> ALTQSVGGDSSADRLFPPQW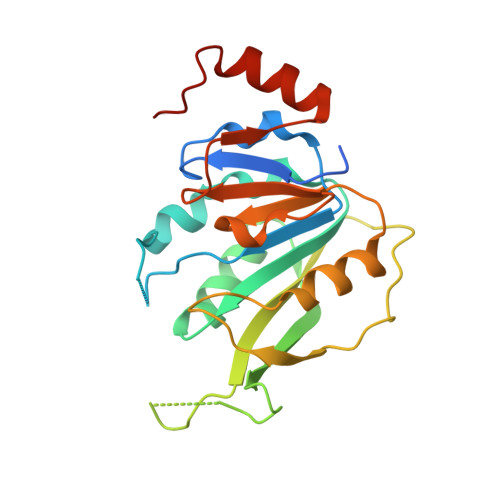ICCDIRYLDVSILGKFAVVMADPPWDIHMELPYGTLTDDEMRRLNIPVLQDDGFLFLWVTGRAMELGRECLNLWGYERVDEIIWVKTNQLQRIIRTGRTGHWLNHGKEHCLVGVKGNPQGFNQGLDCDVIVAEVRSTSHKPDEIYGMIERLSPGTRKIELFGRPHNVQPNWITLGNQLDGIHLLDPDVVARFKQRYPDGIISKPKNL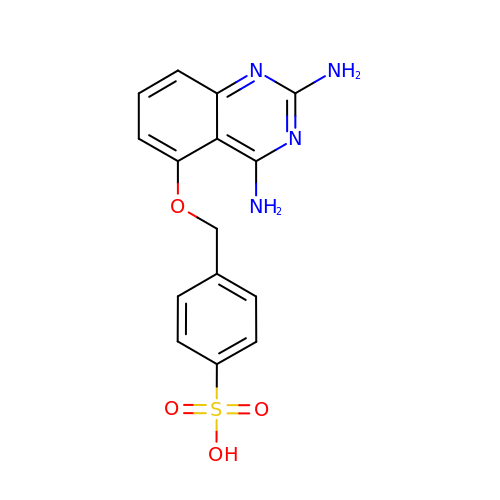4-{[(2,4-diaminoquinazolin-5-yl)oxy]methyl}benzenesulfonic acid | C15 H14 N4 O4 S | AVKNBINNLVQZGS-UHFFFAOYSA-N In bacteria, expression of folate-related genes is controlled by the tetrahydrofolate (THF) riboswitch in response to specific binding of THF and its derivatives. Recently, a second class of THF riboswitches, named THF-II, was identified in Gram-negative bacteria, which exhibit distinct architecture from the previously characterized THF-I riboswitches found in Gram-positive bacteria. Distinct from the aptamers of the previous THF-I riboswitch found in Gram-positive bacteria, the THF-II riboswitch aptamer adopts a simple architecture in which the secondary structure consists of two helices of P1 and P2, two junctions of J12 and J21, and an apical loop L2. The RNA in the ligand–RNA complexes adopts a long rod-like, continuously stacked helix structure stabilized by two helices of P1 and P2 and the interconnecting ligand-bound binding pocket.

We solved the structure with the SAD phasing method by collecting the anomalous signal from Se-urea-soaked crystals. Previously, Se-urea has been utilized to provide an anomalous signal for the SAD phasing of proteins and DNA crystals, but its applicability for RNA crystals has not been tested. By collecting X-ray diffracting data of Se-urea-soaked RNA crystals, we located four Se-urea molecules, which provide strong anomalous signals enough for initial model building. All these four Se-urea molecules interact with RNA by forming hydrogen bonds via the selenium atoms. Their occupancies are 41, 34, 32 and 40%, respectively. The root mean square differentiation (RMSD) between the Se-urea-soaked crystal structure and the native structure is 0.4 Å.

> GGCGUGGUCCGUUCAACUCGUUCCUCGAAAGAGGAACUACGGGAGACGCC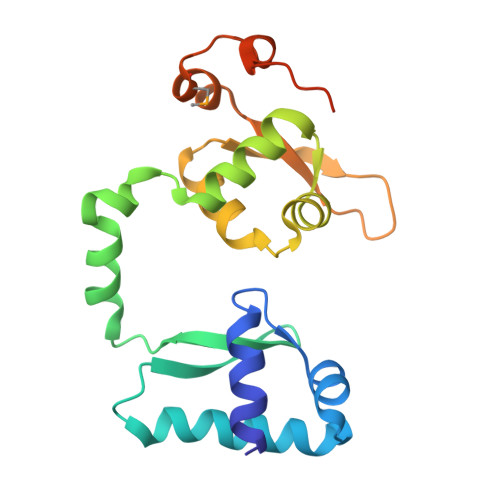> MSTLAKIEALLFVAGEDGIRVRQLAELLSLPPTGIQQSLGKLAQKYEKDPDSSLALIETSGAYRLVTKPQFAEILKEYSKAPINQSLSRAALETLSIIAYKQPITRIEIDAIRGVNSSGALAKLQAFDLIKEDGKKEVLGRPNLYVTTDYFLDYMGINHLEELPVIDELEIQAQESQLFGERI> MIKVEIKPSQAQFTTRSG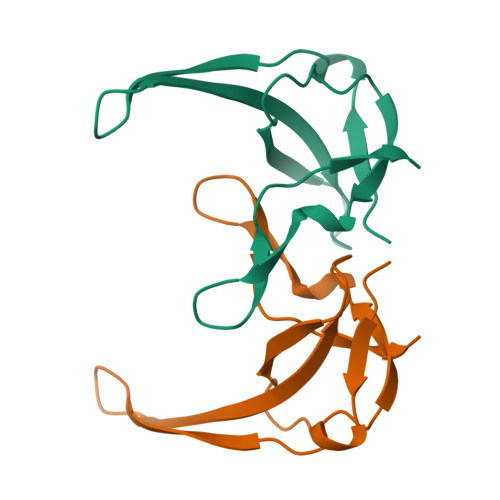VSRQGKPYSLNEQLCYIDLGNEYPVLVKVTLDEGQPAYAPGLYTVHLSSFKVGQFGSLMIDRLRLVPAK> MIKVLFFAQVRELVGTDATEVAADFPTVEAL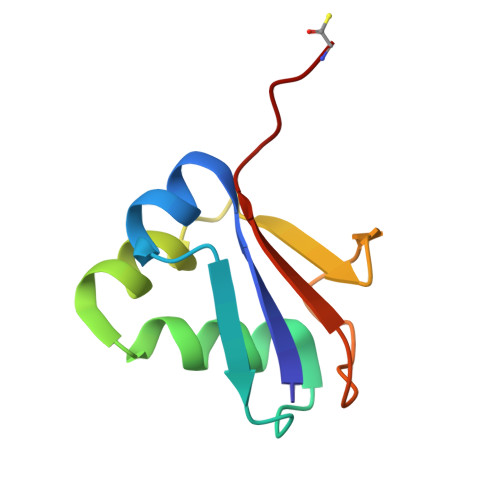RQHMAAQSDRWALALEDGKLLAAVNQTLVSFDHPLTDGDEVAFFPPVTGG>[2x]MSDPTHLISKRAAGRTSVHFTNAPSDKPPANFKPHEKPLALSYGMPNHGFFPIDSIDVNLVDYPFQKITTPSTTSSTAEEEPPSSSLNGSENGHQTKTPPSSIHTPQSTVHISRHTTDPKLIDLARGLQYAAVEGHAPLLQFARDFIIRTHKPNYDDWNVFITTGASDGLNKAADVFLDDGDVILVEEFTFSPFLRFSDNAGAKAVPVKINFDNDSDGIDLTQFVDLLENWEKHYPNLPKPKALYTIATGQNPTGFTQSLEFRKKIYDLAVKYDFAIIEDDPYGYL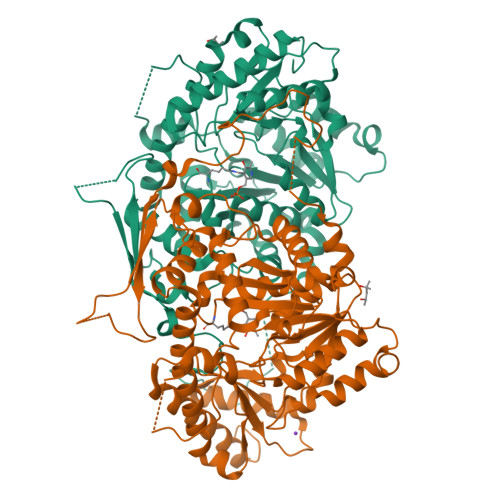TLPKYEKPNIGGSGSGNNELKNDLEIDDYLKNHLTPSYLELDTTGRVLRVETFSKLFAPGLRLGFIVGHKEVIDAVKNYSDVVNRGASGLTQTIVNNVIQENFKGVDGWLEWILKMRLNYSYRKDLLLYSIFESQAYKKGYVDVIDPKAGMFVTFKINLPKDVDVLQKMKLLLWKLISYGILVVPGYNMTVDLEFSKDRSNFFRLCYALANNDEEILESGKRLTDAVYEFFSNGLEFHHHHHH> GSHMIQAYLGLGSNIGDRESQLNDAIKILNEYDGISVSNISPIYETAPVGYTEQPNFLNLCVEIQTTLTVLQLLECCLKTEECLHRIRKERWGPRTLDVDILLYGEEMIDLPKLSVPHPRMNERAFVLIPLNDIA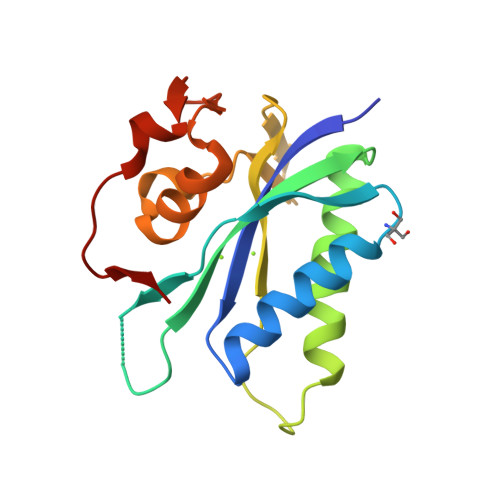ANVVEPRSKLKVKDLVFVNDSVKRYK;>[3x]GSHMIQAYLGLGSNIGDRESQLNDAIKILNEYDGISVSNISPIYETAPVGYTEQPNFLNLCVEIQTTLTVLQLLECCLKTEECLHRIRKERWGPRTLDVDILLYGEEMIDLPKLSVPHPRMNERAFVLIPLNDIAANVVEPRSKLKVKDLVFVDDSVKRYK>GAAASIQTTVNTLSERISSKLEQEANASAQTKCDIEIGNFYIRQNHGCNLTVKNMCSADADAQLDAVLSAATETYSGLTPEQKAYVPAMFTAALNIQTSVNTVVRDFENYVKQTCNSSAVVDNKLKIQNVIIDECYGAPGSPTNLEFINTGSSKGNCAIK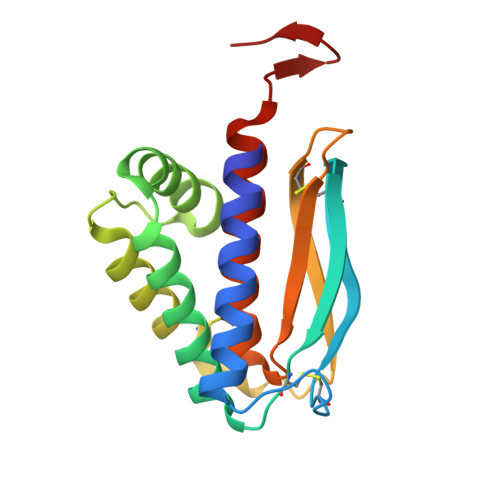ALMQLTTKATTQIAPKQVAGTGVQ[2x]> HMSPSPVPGSQNVPAPAVKKISQYACQRRTTLNNYNQLFTDALDILAENDELRENEGSCLAFMRASSVLKSLPFPITSMKDTEGIPCLGDKVKSIIEGIIEDGESSEAKAVLNDERYKSFKLFTS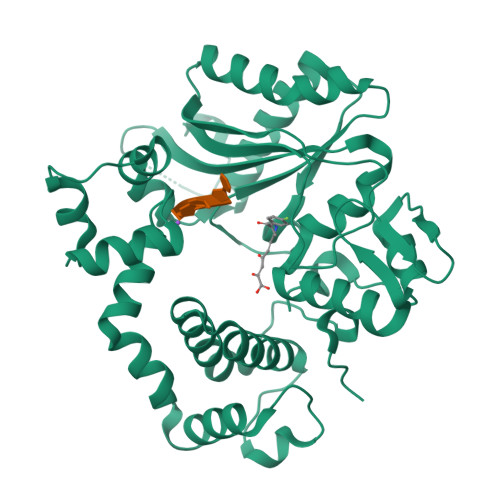VFGVGLKTAEKWFRMGFRTLSKIQSDKSLRFTQMQKAGFLYYEDLVSCVNRPEAEAVSMLVKEAVVTFLPDALVTMTGGFRRGKMTGHDVDFLITSPEATEDEEQQLLHKVTDFWKQQGLLLYCDILESTFEKFKQPSRKVDAADHFQKCFLILKLDHGRVHSEKSGQQEGKGWKAIRVDLVMCPYDRRAFALLGWTGSRQFERDLRRYATHERKMMLDNHALYDRTKRVFLEAESEEEIFAHLGLDYIEPWERNA>MNPIVINRLQRKLGYTFNHQELLQQALTHRSASSKHNARLEFLGDSILSYVIANALYHRFPRVDAGDMSRMRATLVRGNTLAELAREFELGECLRLGPGELKSGGFRRESILADTVEALIGGVFLDSDIQTVEKLILNWYQTRLDEISPGDKQKDPKT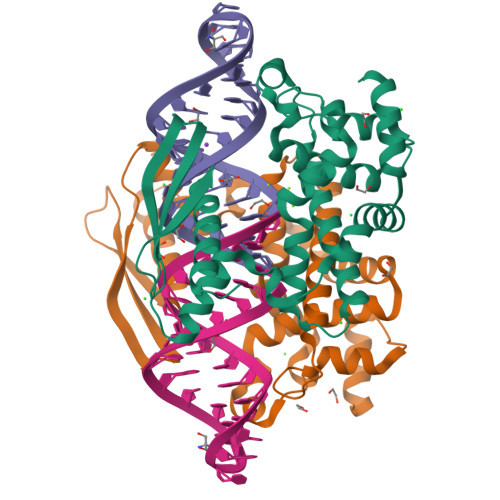RLQEYLAGRHLPLPTYLVVQVRGEAHDQEFTIHCQVSGLSEPVVGTGSSRRKAEQAAAEQALKKLELE[2x]> MSTPAV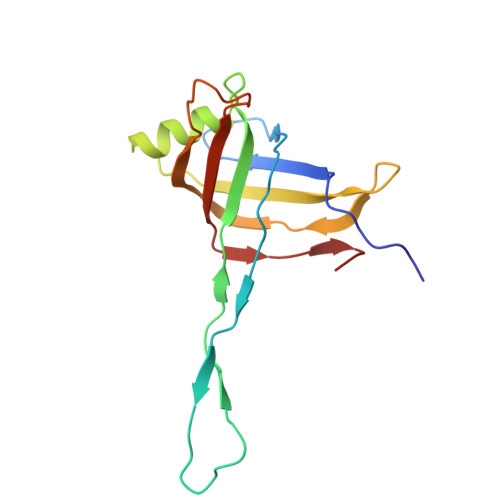SHRFLVNFLFNNIPNPFDIAFQRISGLSRTLEVSQHREGGENVRNLWLAEQVNHGSLVLERGVMNASPLTLQFDRVLRRESTQWANVVIMLLNELSLPVTTWTLSHALPVRWQMGDLDAGSNQVLINTLELRYQDMRMLGVKL>GSLIGTTAKVNRIREITAAKMVEALQISAQLTHLQEVDMTKIAELRKESKPAFQQKYGVNLTYLPFFVKAAVEALVSHPNVNASYNAETKEMTYHADVNVAIAVDTPRGLLTPVIHKAQELTFPEIAQAIVDLADRARNNKLKPQDLMGATFTITNIGSEGALSDTPILVPPQAGILGTAAIQKRAVVVTEDGVDAIAIRQMCYMPFTYDHQVVDGADAGRFT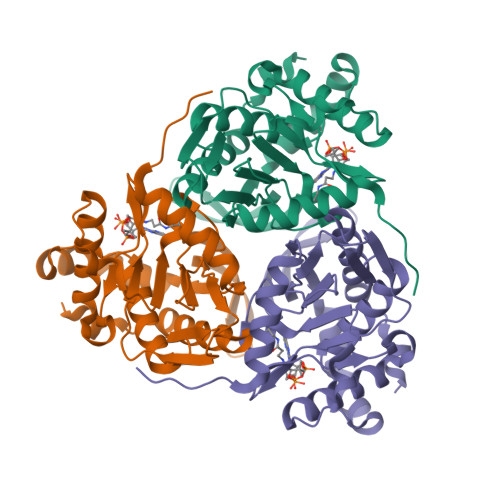TTIKDRLETANFADDLAL[2x]>TTIVSVRRNGHVVIAGDGQATLGNTVMKGNVKKVRRLYNDKVIAGFAGGTADAFTLFELFERKLEMHQGHLVKAAVELAKDWRTDRMLRKLEALLAVADETASLIITGNGDVVQPENDLIAIGSGGPYAQAAARALLENTELSAREIAEKALDIAGDICIYTNHFHTIEELSYKA[4x];>HHHHHHHSEMTPREIVSELDKHIIGQDNAKRSVAIALRNRWRRMQLNEELRHEVTPKNILMIGPTGVGKTEIARRLAKLANAPFIKVEATKFTEVGYVGKEVDSIIRDLTDAAVKMVRVQAIEKNRYRAEELAEERILDVLIPPAKNNWGQTEQQQEPSAARQAFRKKLREGQLDDKEIEIDLAAAPMGVEIMAPPGMEEMTSQLQSMFQNLGGQKQKARKLKIKDAMKLLIEEEAAKLVNPEELKQDAIDAVEQHGIVFIDEIDKICKRGESSGPDVSREGVQRDLLPLVEGCTVSTKHGMVKTDHILFIASGAFQIAKPSDLIPELQGRLPIRVELQALTTSDFERILTEPNASITVQYKALMATEGVNIEFTDSGIKR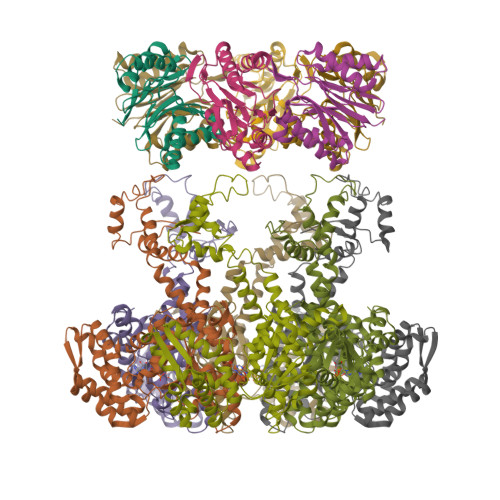IAEAAWQVNESTENIGARRLHTVLERLMEEISYDASDLSGQNITIDADYVSKHLDALVADEDLSRFIL[2x]> QKPGETKEVHPQLTTFRCTKRGGCKPATNFIVLDSLSHPIHRAEGLGPGGCGDWGNPPPKDVCPDVESCAKNCIMEGIPDYSQYGVTTNGTSLRLQHILPDGRVPSPRVYLLDKTKRRYEMLHLTGFEFTFDVDATKLPCGMNSALYLSEMHPTGAKSKYNPGGAYYGTGYCD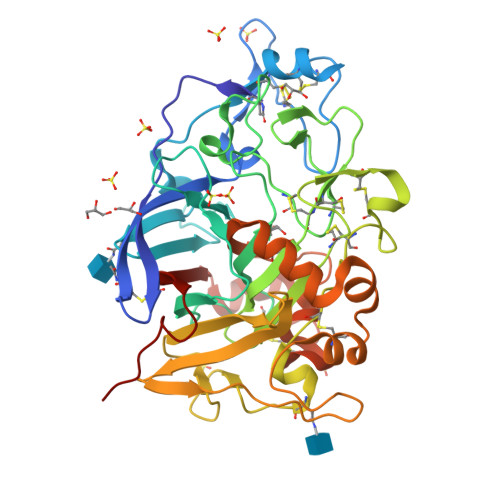AQCFVTPFINGLGNIEGKGSCCNEMDIWEANSRASHVAPHTCNKKGLYLCEGEECAFEGVCDKNGCGWNNYRVNVTDYYGRGEEFKVNTLKPFTVVTQFLANRRGKLEKIHRFYVQDGKVIESFYTNKEGVPYTNMIDDEFCEATGSRKYMELGATQGMGEALTRGMVLAMSIWWDQGGNMEWLDHGEAGPCAKGEGAPSNIVQVEPFPEVTYTNLRWGEIGSTYQELQ> MISTTISGKRPIEQVDDELLSLTAQQENEEQQQQRKRRRHQFAPMTQFNSNTLDEDSGFRSSSDVATADQDNFLEESPSGYIKKVILRNFMCHEHFELELGSRLNFIVGNNGSGKSAILTAITIGLGAKASETNRGSSLKDLIREGCYSAKIILHLDNSKYGAYQQGIFGNEIIVERIIKRDGPASFSLRSENGKEISNKKKDIQTVVDYFSVPVSNPMCFLSQDAARSFLTASTSQDKYSHFMKGTLLQEITENLLYA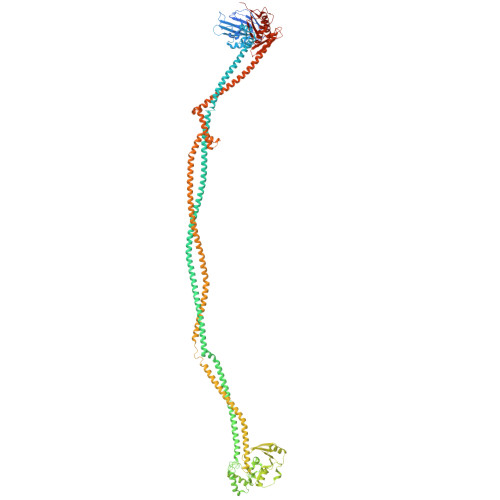SAIHDSAQENMALHLENLKSLKAEYEDAKKLLRELNQTSDLNERKMLLQAKSLWIDVAHNTDACKNLENEISGIQQKVDEVTEKIRNRQEKIERYTSDGTTIEAQIDAKVIYVNEKDSEHQNARELLRDVKSRFEKEKSNQAEAQSNIDQGRKKVDALNKTIAHLEEELTKEMGGDKDQMRQELEQLEKANEKLREVNNSLVVSLQDVKNEERDIQHERESELRTISRSIQNKKVELQNIAKGNDTFLMNFDRNMDRLLRTIEQRKNEFETPAIGPLGSLVTIRKGFEKWTRSIQRAISSSLNAFVVSNPKDNRLFRDIMRSCGIRSNIPIVTYCLSQFDYSKGRAHGNYPTIVDALEFSKPEIECLFVDLSRIERIVLIEDKNEARNFLQRNPVNVNMALSLRDRRSGFQLSGGYRLDTVTYQDKIRLKVNSSSDNGTQYLKDLIEQETKELQNIRDRYEEKLSEVRSRLKEIDGRLKSTKNEMRKTNFRMTELKMNVGKVVDTGILNSKINERKNQEQAIASYEAAKEELGLKIEQIAQEAQPIKEQYDSTKLALVEAQDELQQLKEDINSRQSKIQKYKDDTIYYEDKKKVYLENIKKIEVNVAALKEGIQRQIQNACAFCSKERIENVDLPDTQEEIKRELDKVSRMIQKAEKSLGLSQEEVIALFEKCRNKYKEGQKKYMEIDEALNRLHNSLKARDQNYKNAEKGTCFDADMDFRASLKVRKFSGNLSFIKDTKSLEIYILTTNDEKARNVDTLSGGEKSFSQMALLLATWKPMRSRIIALDEFDVFMDQVNRKIGTTLIVKKLKDIARTQTIIITPQDIGKIADIDSSGVSIHRMRDPERQNNSNFYN> GAMGRSVYELDCIPLWGTVSIQGNRSEMEDAFAVSPHFLKLPIKMLMGDHEGMSPSLTHLTGHFFGVYDGHGGHKVADYCRDRLHFALAEEIERIKDELCKRNTGEGRQVQWDKVFTSCFLTVDGEIEGKIGRAVVGSSDKVL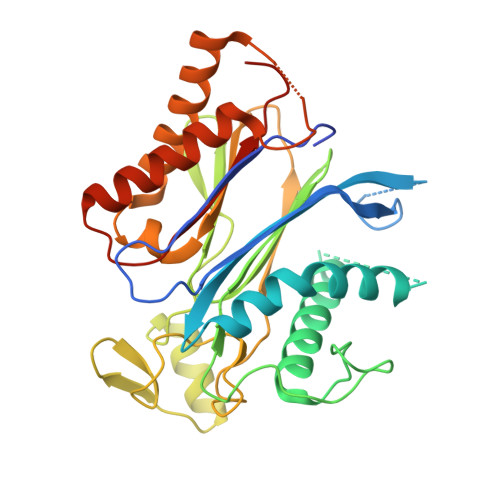EAVASETVGSTAVVALVCSSHIVVSNCGDSRAVLFRGKEAMPLSVDHKPDREDEYARIENAGGKVIQWQGARVFGVLAMSRSIGDRYLKPYVIPEPEVTFMPRSREDECLILASDGLWDVMNNQEVCEIARRRILMWHKKNGAPPLAERGKGIDPACQAAADYLSMLALQKGSKDNISIIVIDLKAQRKFKTRT> GSHMKNVSGSVKLWVDTTQVPYYKKIVANFNKKYPDVKVKVTQSPNGSANAKTDVGKDPAKAADVFEVANDQLGSMAEAGYINPLSPDATKAVKNNNVAVASEGVTWKGKMFAYPFAEQAQTIYYNKSKLTADDVKTWDGLTAKGVLATDFTNAYNFYPVFLSAGTQLYGKTGETVKGTDVNSAKGEQAMAWFAQQKSNKGVMQTSNALNQLKSGKAAAILDGPWNSANIKKILGKNFAVAPYPTIKLDGKDVQMQAFLGIETFAVNSHASGSNQKAAATLASFITNKESQLIVYDHSGQIPVDKTAQKSSKVASDPVAGAVMTMAKPGNSTLMPKMPQMATFWNDAAPLINGA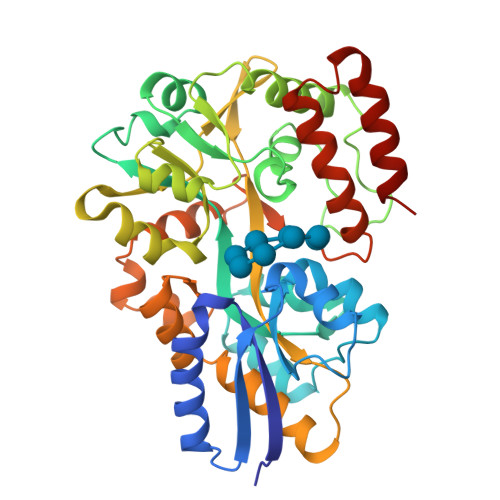YTGSIPASQYSTKLDTFVKNISKAN> MGSMTTDLDTLSDQLRKNYYRDLSLFQDDEDPFYHYLI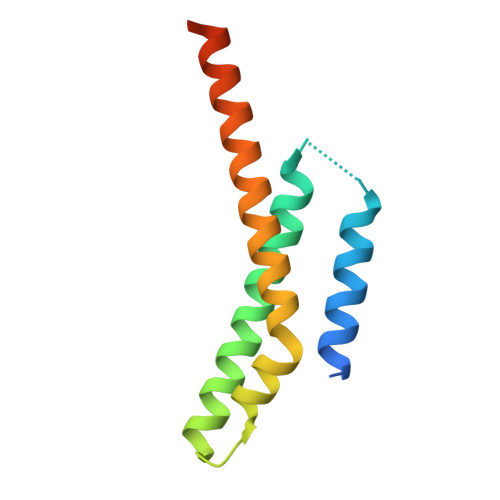STKLATNLNTVRKLAIKDNLDDPSSDAIDRYQKNFSRLEESVSSISFSKASKLQQKYDAYQESQKKRRYSVDFDA> DCAKEGEVCSWGKKCCDLDN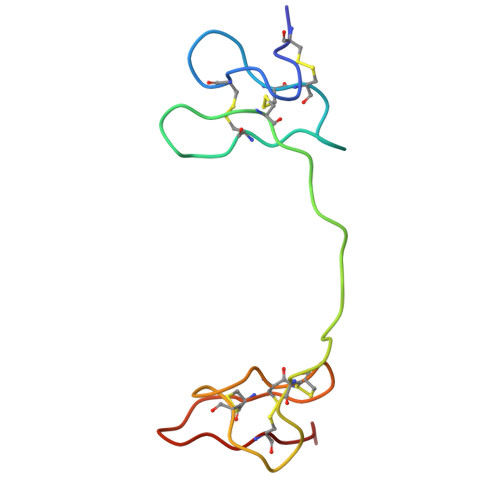FYCPMEFIPHCKKYKPYVPVTTNCAKEGEVCGWGSKCCHGLDCPLAFIPYCEKYR> GAMEFERAKAAVESDTEFWDKMQAEWEEMARRNWISENQEAQNQVTVSASEKGYYFHTENPFKDWPGAFEEGLKRLKEGDLPV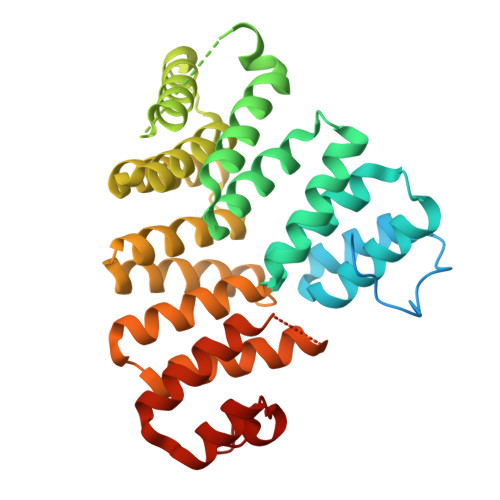TILFMEAAILQDPGDAEAWQFLGITQAENENEQAAIVALQRCLELQPNNLKALMALAVSYTNTSHQQDACEALKNWIKQNPKYKYLVKNKKGSPGLTRRMSKSPVDSSVLEGVKELYLEAAHQNGDMIDPDLQTGLGVLFHLSGEFNRAIDAFNAALTVRPEDYSLWNRLGATLANGDRSEEAVEAYTRALEIQPGFIRSRYNLGISCINLGAYREAVSNFLTALSLQRKSRNQQQVPHPAISGNIWAALRIALSLMDQPELFQAANLGDLDVLLRAFNLDP> FSIVGT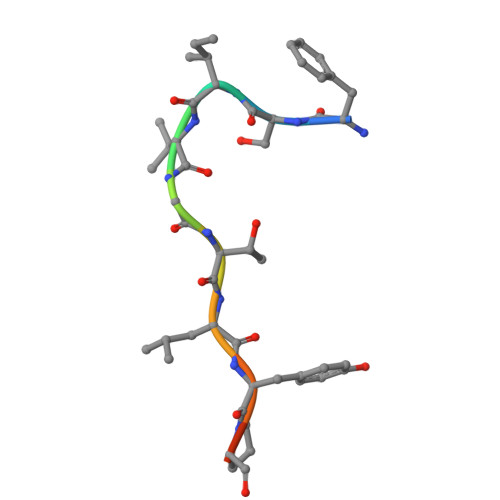LYPIN> MHHHHHHSTATNPLDLDVCAREPIHIPGLIQPYGVLLVIDPADGRIVQASTTAADLLGVPMAALLGMPYTQVLTLPEAQPFAVDDQPQHLMHAEVRFPQRATPPASAWVAAWHLYPQQWLVEMEPRDARLLDVTLREAMPLLRSVERDPGIAEAAVRVAKGLRSLIGFDRVMIYRFDEEWNGDIIAEARKPELEAYLGLHYPASDIPAQARALYLRNRVRQIADVGYQPSP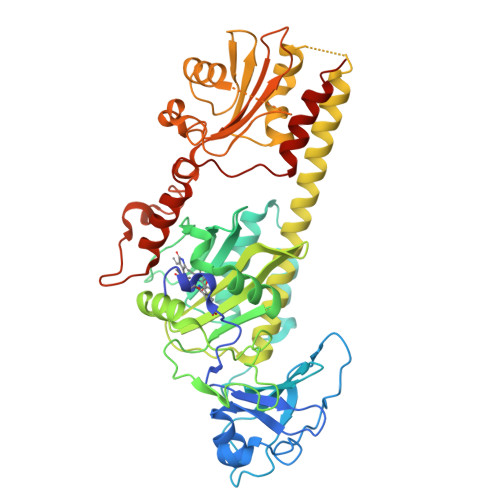IQPTVHPQLGTPVDLSDVSLRSVSPVHLEYLANMGVTATLVASIVVNDALWGLISCHHYSPHFTNHAMRDVTDAVARTLAGRIGALQAVARARLESVLLTVREKLITDFNDAEHMTVELLDDMAPDLMDVVDADGVAIFHGNDISRHGTTPDVAALRRIRDHIESEHHEALREDAVGALHVDAIGEVFPELADLAPLAAGFIFVPLMPQSRSALLWTRREQIQQIKWAGNPQLAKLEDIPNSRLSPRKSFDLWQQTVRGRARRWSPLHLESARSLRVLIELMERKR> GAVQNDEVAAFCQSIMKLKTKFPYTDHCTNPGYLLSPVTVQRNMCGENASVKVSIEIEGLQLPVTFTCDVSSTVEIIIMQALCWVHDDLNQVDVGSYILKVCGQEEVLQNNHCLGSHEHIQNCRKWDTEIKLQLLTLSAMCQNLARTAEDDEAPVDLNGSGSVMTRHPVEELLDSYHYQVELALQTENQHRAVDQVIKAVRKICSALDGVETPSVTEAVKKLKRAVNLPRNKSADVTSLSGSDTRKNSTKGSLNPENPVQVSMDHLTTAIYDLLRLHANSSRCSTGCPRGSRNIKEAWTATEQLQFTVYAAHGISSNWVSNYEKYYLICSLSHNGKDLFKPIQSKKVGTYKNFFYLIKWDELIIFPIQISQLPLESVLHLTLFGVLNQSSGSSPDSNKQRKGPEALGKVSLTLFDFKRFLTCGTKLLYLWTSSHTNSIPGAIPKKSYVMERIVLQVDFPSPAFDIIYTSPQIDRNIIQQDKLETLESDIKGKLLDIIHRDSSFGLSKEDKVFLWENRYYCLKHPNCLPKILASAPNWKWANLAKTYSLLHQWPPLCPLAALELLDAKFADQEVRSLAVSWMEAISDDELADLLPQFVQALKYEIYLNSSLVRFLLSRALGNIQIAHSLYWLLKDALHDTHFGSRYEHVLGALLSVGGKGLREELSKQMKLVQLLGGVAEKVRQASGSTRQVVLQKSMERVQSFFLRNKCRLPLKPSLVAKELNIKSCSFFSSNAMPLKVTMVNADPLGEEINVMFKVGEDLRQDMLALQMIKIMDKIWLKEGLDLRMVIFRCLSTGRDRGMVELVPASDTLRKIQVEYGVTGSFKDKPLAEWLRKYNPSEEEYEKASENFIYSCAGCCVATYVLGICDRHNDNIMLRSTGHMFHIDFGKFLGHAQMFGSFKRDRAPFVLTSDMAYVINGGEKPTIRFQLFVDLCCQAYNLIRKQTNLFLNLLSLMIPSGLPELTSIQDLKYVRDALQPQTTDAEATIFFTRLIESSLGSIATKFNFFIHNLAQLRFSGLPSNDEPILSFSPKTYSFRQDGRIKEVSVFTYHKKYNPDKHYIYVVRILREGHLEPSFVFRTFDEFQELHNKLSIIFPLWKLPGFPNRMVLGRTHIKDVAAKRKIELNSYLQSLMNASTDVAECDLVCTFFHPLLRDEK

Phosphatidylinositol 3-kinase type 2α (PI3KC2α) is an essential member of the structurally unresolved class II PI3K family with crucial functions in lipid signaling, endocytosis, angiogenesis, viral replication, platelet formation and a role in mitosis. The class II PI3K isoforms PI3KC2α, PI3KC2β and PI3KC2γ are unique in directly synthesizing PI 3,4-bisphosphate (PI(3,4)P2) from PI 4-phosphate (PI(4)P) at the plasma membrane and within the endolysosomal system, in addition to synthesis of PI 3-phosphate (PI(3)P). Like other members of the PI3K family, PI3KC2α contains a PI3K core that consists of a Ras-binding domain (RBD) and an N-terminal C2 domain, as well as helical and kinase domains (KDs). In addition, PI3KC2α harbors the C-terminal Phox-homology (PX) and C2 domains that are unique to class II enzymes.

To determine the X-ray crystal structure of PI3KC2α, we embarked on an iterative process of construct screening and optimization of various forms of PI3KC2α from different species assisted by hydrogen/deuterium exchange–mass spectrometry (HDX–MS) to identify disordered regions. A purified mouse PI3KC2α construct containing a re-engineered internal loop sequence and lacking the intrinsically disordered N-terminal region and the C-terminal C2 domain (C-C2) was used to obtain the 3.3 Å crystal structure of PI3KC2αΔN+ΔC−C2. The overall structure of PI3KC2αΔN+ΔC−C2 comprises a large compact multidomain kinase core that is mounted onto a helical stalk. A conserved feature of all mammalian class II PI3Ks is a sequence insertion of about 100 amino acids between the RBD and the N-C2 domain that is absent in class I and class III enzymes. This sequence folds into a unique stalk-forming HBD comprising four helices. The compact core region is flanked by the distantly located PX domain that is stabilized by contacts with a neighboring molecule in the crystal. The release of the PX-C2 domain from the catalytic core may thus indicate that the obtained PI3KC2αΔN+ΔC−C2 crystal structure represents an active conformation of the enzyme, a hypothesis tested and corroborated below. Consistently, we observed the PX domain to be displaced from the kinase core, and closed contact I involving the N terminus of kα12 to be disrupted in the crystal structure of PI3KC2αΔN+ΔC−C2. Instead, in this open conformation of PI3KC2α, the kα12 helix interacts via hydrogen bonding of H1391 with the backbone of a short helical segment within the intermediate section of the activation loop. Torin-2 binds to PI3KC2α in a mode similar to mTOR.>[2x]MKRMEANKIKLINEDNLRLDGRSFNELRPIKIQAGVLNRADGSAYIEWGGNKIMVGVYGPKEAYPKHSQDIDHAIVKARYNMAAFSVDERKRPGPDRRTMEISKVISEALSSSIMIEQFPRAEIDVYIEVLQADAGTRIAGLTAATVALADAGVPMRDMVVGCTAGKVDGHMVLDLSKEEDNYGEADIPIAIMPKTGDIVLMQMDGDVTEDELYQAMDMIFEATKRISQIQREALLNKYKIQDIGEGEMVKESAEILSEIRKNYILSTMKGGKRIDGRLPDEFRELTIIENYIPRANGSAYVALGNTRVVAGVKIEAGEPFPDTPDQGVLTTNVELLPIAFPSFEAGPPNDLAIEVSRVVDRGIRESKMISPEKLVIEQGKKVWIVFLDINVLDYDGNLIDASTIAAVAALRNAVVPASKEGGEDFKLPVSSTPISVTMVKIGDTLVCDPSLEEDQICGGRITVTTTEDGHIRAMQKGEIGAFTVEDVKKAVKMSLEVGKKLREKYFR

The exosome is a multiprotein complex that participates in the processing and degradation of RNA molecules. Several studies have linked exosomes to the quality control of messenger RNA (mRNA), the turnover of cytosolic messenger RNA (mRNA), and the processing of short noncoding RNA (sncRNA). Archaeal exosomes, unlike those of eukaryotes, contain only two RNase-PH-like subunits, Rrp41 and Rrp42. These subunits form a hexameric ring where Rrp41 and Rrp42 exist as heterodimers.

The crystal structure of TaciRrp41:42 with a phosphate ion was solved at 2.3 Å and belonged to the P213 space group. The TaciRrp41 and TaciRrp42 structural component revealed a heterodimeric complex structure of the exosome core at 2.3 Å. The overall exosome structure of Taci consists of nine subunits, three TaciRrp41 and TaciRrp42 heterodimers forming a hexameric ring structure and capped on one side by three subunits of TaciRrp4. Both TaciRrp41 and TaciRrp42 have an RNase-PH-like fold, with the characteristic of β-α-β layers of secondary structure elements. When the TaciRrp41 and TaciRrp42 subunits combine to form a complex, it was observed that the ninth β strands of each subunit aligned in an anti-parallel manner. Consequently, a total of eight β strands from each subunit were arranged in an anti-parallel structure. Also, four salt bridges were found to contribute to the stabilization of dimerization. The three salt bridges were located between helices surrounding the eight β strands (210E41–245K42, 104K41–107E42, 101E41–110R42), while the remaining one was formed between a TaciRrp42 β strand and a TaciRrp41 loop (207D41–225R42) (the superscripts 41 and 42 stand for TaciRrp41 and TaciRrp42, respectively). The central chamber within the ring contains three phosphorolytic active sites located at the interface between TaciRrp42 and TaciRrp41. Furthermore, many arginine residues from TaciRrp41 and TaciRrp42 are involved in forming a positively charged region around the inorganic phosphate. When superimposed on this structure, the position of the P1 phosphate coincided with the phosphate-binding site of S. sol.>GSAE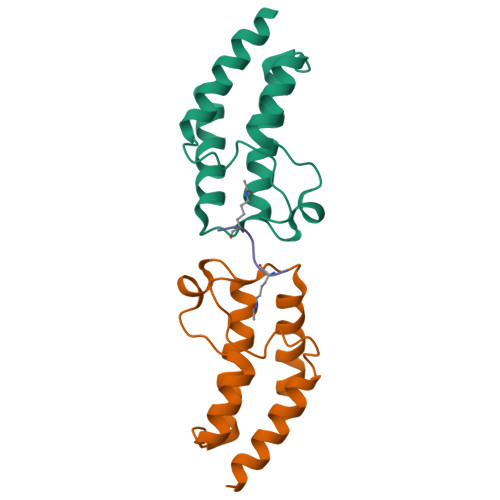NESTPIQQLLEHFLRQLQRKDPHGFFAFPVTDAIAPGYSMIIKHPMDFGTMKDKIVANEYKSVTEFKADFKLMCDNAMTYNRPDTVYYKLAKKILHAGFKMMSK[4x];>[2x]SGRGKGGKGLG>GMEPITQAFAQQFSREWIDAWNAHDLDAILSHYADGFEMSSPMIVQIAGEPSGRLRGKEQVGAYWREALRMIPDLH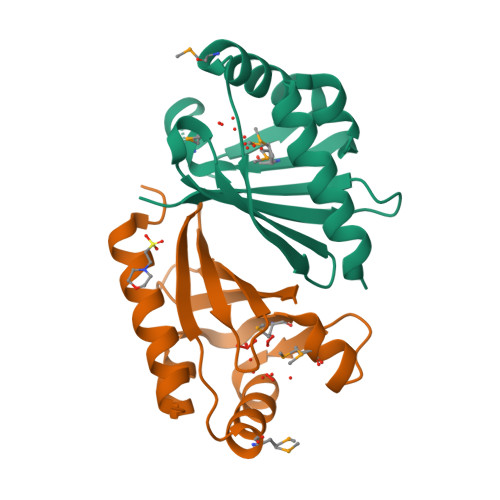FEWIATLAGVDSVAIHYRGAKGRLALEVFHFGPDRRVVKALAHYAG[2x]VhChiP is a chitooligosaccharide-specific porin identified in the outer membrane of Vibrio campbellii type strain American Type Culture Collection BAA 1116. VhChiP contains three identical subunits, and in each subunit, the 19-amino acid N-terminal segment serves as a molecular plug (the “N-plug”) that controls the closed/open dynamics of the neighboring pores. VhChiP is a sugar-specific OM porin with the ability to selectively transport a range of chitooligosaccharides, chitohexaose being the most preferred. VhChiP consists of three identical β-barrels, each containing 16 β-strands connected on the extracellular side by eight hydrophilic loops and on the periplasmic side by eight short hydrophobic turns.

The N-plug peptide corresponding to the first nine residues (DGANSDAAK) inside the protein pore was synthesized and added on either cis or trans side of the sample cell partitioned by the lipid bilayer, and its effects on the binding kinetics of sugar–channel interactions were investigated. Under the applied potential of +100 mV in 1 M KCl, 20 mM Hepes, pH 7.4, rare and short-lived blocking events were observed when the truncated channel was exposed to the N-plug peptide at 10 and 40 μM. The results were markedly different with the addition of chitohexaose on the cis side and the N-plug peptide on the trans side. Strong blocking events at a monomeric level from state O3 (fully open) to O2 (one monomer closure) were observed with 10 μM N-plug peptide added. When chitohexaose was added on the cis and N-plug on the trans side, the K value returned to 255,000 M−1, the value for chitohexaose–WT channel interactions. Titration of chitohexaose into the truncated channel yielded a Kd of 10 ± 0.3 μM and a stoichiometry of 2.8 ± 0.1, while titration of chitohexaose with the truncated VhChiP mixed with the N-plug peptide yielded a Kd of 2.9 ± 0.07 μM and a stoichiometry of 2.3 ± 0.2.

>EVYGIIAMQAAYRDYDSGDAKQDDNLGGMQLNNESRIGFRGKKQFANFEPTFIWQIEGGYVDPSFGGEGAGLGERDTFVGFESASWGQVRLGRVLTPMYELVDWPASNPGLGDVYDWGGAIGGAKYQDRQSNTIRWDSPMYADKFSIDAAVGAGDKAGLGAGDDYWGGIAAHYKLGPLQLDAAYEGNRNIEAEGQTWENNTYLVGVQGWFENGISFFAQYKYMEADASNGVNEKQDAMSAGLMYTTGDWQYKLGYAANFDLERDGKTLSNTSDDVVSAQIMYFVDPSAVLYARARMNDFNEGLDGLDDAARWTSGTNGDYNEYSVGVEYYF[6x];> DGANSD3-(furan-2-yl)-1-methyl-1H-pyrazole-5-carboxylic acid | C9 H8 N2 O3 | 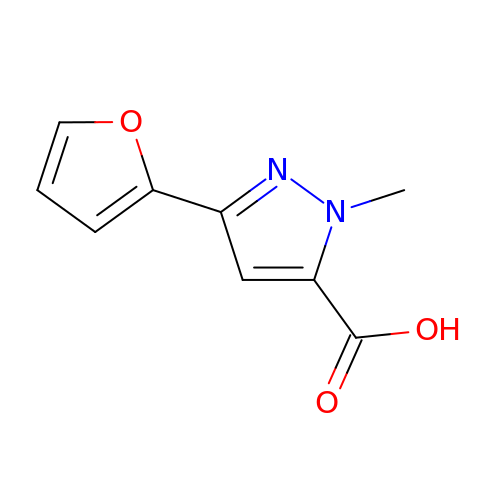MOPCEJWYTICWJM-UHFFFAOYSA-N>[8x]SRQLWKWSGNPTQRRGMKGKARKLFYKAIVRGKETLRIGDCAVFLSAGRPNLPYIGRIESLWESWGSNM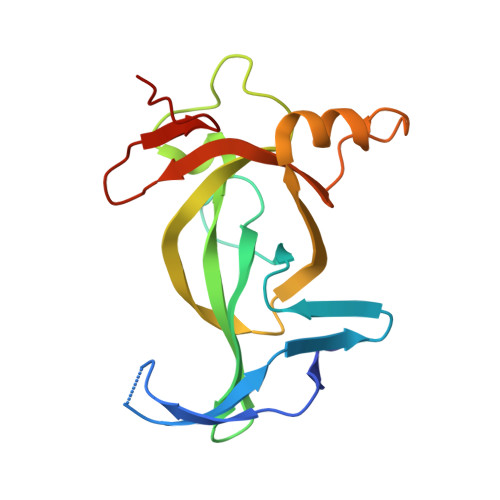VVKVKWFYHPEETKLGKRQSDGKNALYQSCHEDENDVQTISHKCQVVGREQYEQMMRGRKYQDQQDLYYLAGTYDPTTGRLVTADGVPVLC;>[4x]ATKAARKSAPATGW>MTHWSADYGWRGKVGLISTPVIENAHVELARVAPEGVGVYQTFPYVPNFRVDATNIKRAVEQLETSAAALGSAGVDIVGQVGTPFSFAGGTGLEWAEDISTKLEKASGKPVA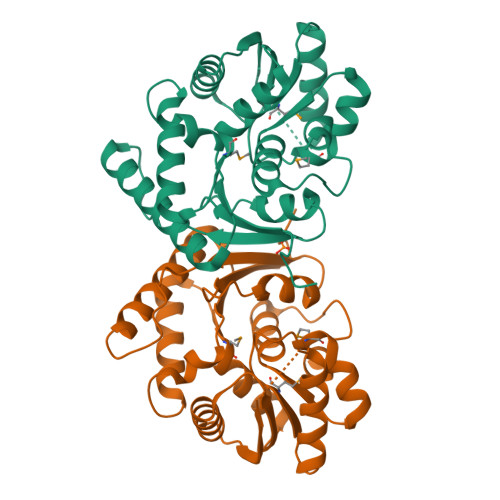LMGLSIVEALQERGYKTVAISSTYYSRELSERYTQFLEAGGIRVLTIKNWVDQKRFPDEESVDGRNLWYPASYAYKSAREVAAEAPEADCIIMSGAAVHTMDIIAPLEADLGKPVISSDSAFFWKILSLLGVRETSGGWGSLLDSL[8x]> GPVPMHPFVKALQEHFTAHQNPEKAEPMARYMKNHFLFLGIQTPERRQLLKDIIQIHTLPDQKDFQIIIRELWDLPEREFQAAALDIMQKYKKHINETHIPFLEELIVTKSWWDSVDSIVPTFLGDIFLKHPELISAYIPKWIASDNIWLQRAAILFQLKYKQKMDEELLFWIIGQLHSSKE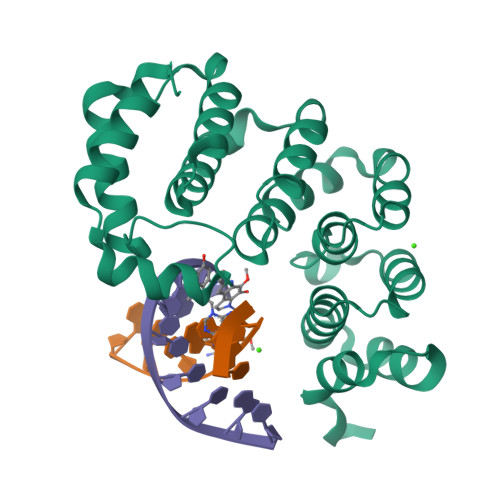FFIQKAIGWVLREYAKTNPDVVWEYVQNNELAPLSKREAIKHIKQNYGINNEKIGETLS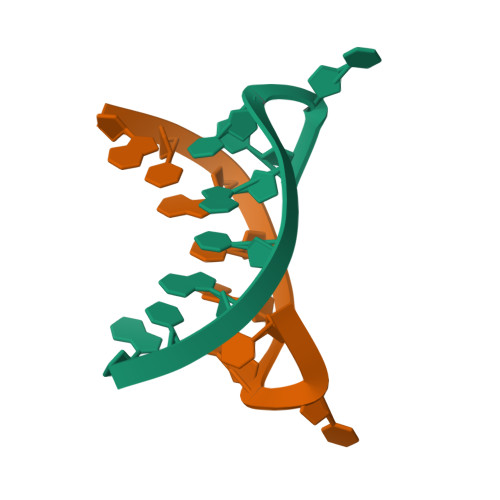>[14x]ATATATCT>[2x]MANGANRVDLDGKPIQPLTICMIGAGGFIGSHLCEKLLTETPHKVLALDVYNDKIKHLLEPDTVEWSGRIQFHRINIKHDSRLEGLVKMADLIINLAAIATPADYNTRPLDTIYSNFIDALPVVKYCSENNKRLIHFSTCEVYGKTIGSFLPKDHPLRDDPAFYVLKEDISPCIFGSIEKQRWSYACAKQLIERLVY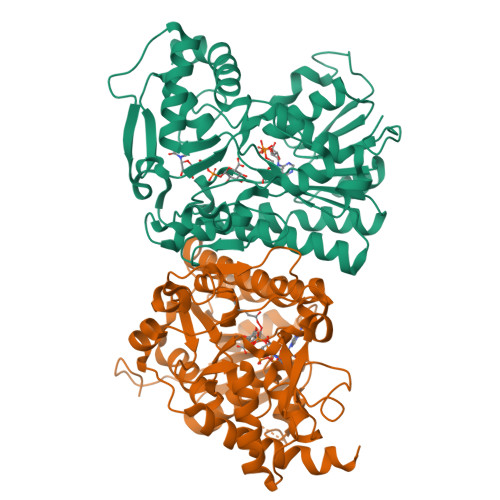AEGAENGLEFTIVRPFNWIGPRMDFIPGIDGPSEGVPRVLACFSNNLLRREPLKLVDGGESQRTFVYINDAIEAVLLMIENPERANGHIFNVGNPNNEVTVRQLAEMMTEVYAKVSGEGAIESPTVDVSSKEFYGEGYDDSDKRIPDMTIINRQLGWNPKTSLWDLLESTLTYQHRTYAEAVKKATSKPVAS> PRGSALSDTERAQLDVMKLLNVSLHEMSRKISRS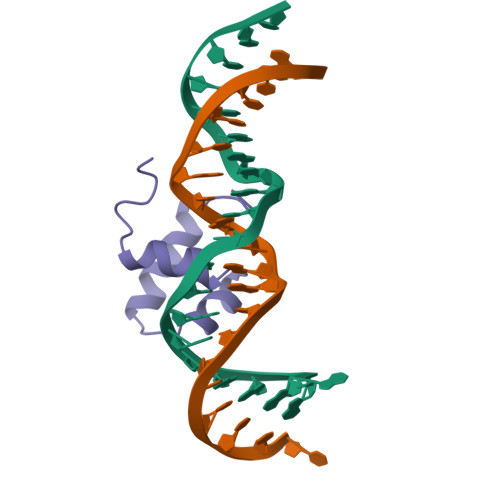RHCIRVYLKDPVSYGTS>MAESEAETPSTPGEFESKYFEFHGVRLPPFCRGKMEEIANFPVRPSDVWIVTYPKSGTSLLQEVVYLVSQGADPDEIGLMNIDEQLPVLEYPQPGLDIIKELTSPRLIKSHLPYRFLPSDLHNGDSKVIYMARNPKDLVVSYYQFHRSLRTMSYRGTFQEFCRRFMNDKLGYGSWFEHVQEFWEHRMDSNVLFLKYEDMHRDLVTMVEQLARFLGVSCD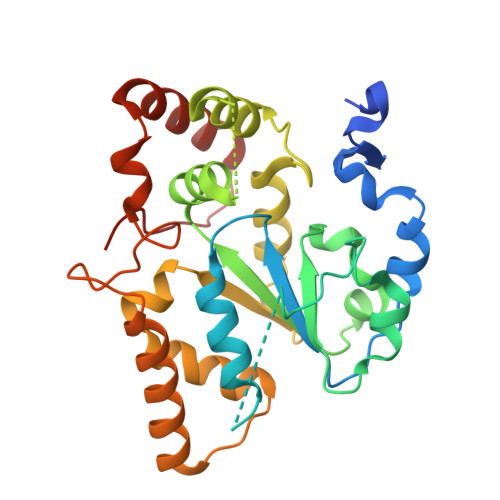KAQLEALTEHCHQLVDQCCNAEALPVGRGRVGLWKDIFTVSMNEKFDLVYKQKMGKCDLTFDFYL[2x]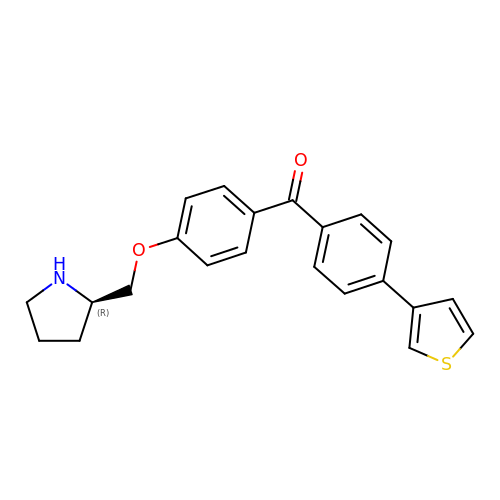{4-[(2R)-pyrrolidin-2-ylmethoxy]phenyl}(4-thiophen-3-ylphenyl)methanone | C22 H21 N O2 S | VUWFJUJWAWMRQN-HXUWFJFHSA-N>[4x]MGSSHHHHHHGSNAWEVNFD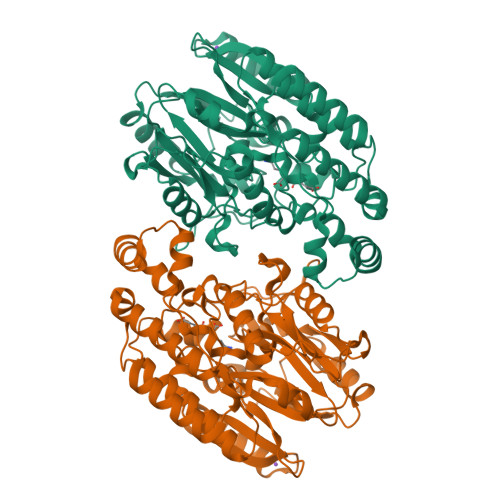GLVGLTHHYAGLSFGNEASTRHRFQVSNPRLAAKQGLLKMKALADAGFPQAVIPPHERPFIPVLRQLGFSGSDEQVLEKVARQAPHWLSSVSSASPMWVANAATIAPSADTLDGKVHLTVANLNNKFHRSLEAPVTESLLKAIFNDEEKFSVHSALPQVALLGDEGAANHNRLGGHYGEPGMQLFVYGREEGNDTRPSRYPARQTREASEAVARLNQVNPQQVIFAQQNPDVIDQGVFHNDVIAVSNRQVLFCHQQAFARQSQLLANLRARVNGFMAIEVPATQVSVSDTVSTYLFNSQLLSRDDGSMMLVLPQECREHAGVWGYLNELLAADNPISELKVFDLRESMANGGGPACLRLRVVLTEEERRAVNPAVMMNDTLFNALNDWVDRYYRDRLTAADLADPQLLREGREALDVLSQLLNLGSVYPFQREGGGNG Non-ribosomal peptide synthetases are important enzymes for the assembly of complex peptide natural products. Within these multi-modular assembly lines, condensation domains perform the central function of chain assembly, typically by forming a peptide bond between two peptidyl carrier protein (PCP)-bound substrates. To address this, we report the structure and biochemical characterization of complexes of a PCP domain bearing a stable analog of the acyl acceptor complexed to the acceptor site of a C domain from the NRPS that biosynthesizes fuscachelin in the thermophile Thermobifida fusca. The C3 domain of the didomain resembles other members of its class, comprising a pseudo-dimer of CAT domains with bridge (R2923 to T2944) and floor loop (A2843 to L2858) regions.

The crystals belonged to the P212121 space group, with the unit cell comprising two highly similar copies of the PCP2-C3 construct (RMSD (all atoms) 0.74 Å). In the PCP2-C3 didomain structure, the PCP2 domain sits at the acceptor-PCP binding site (near the opening of the acceptor substrate channel) on the C3 domain from the second chain in the asymmetric unit. The interface between the PCP2 domain and C3 domain is mostly hydrophobic in nature (537/510 Å2 buried surface area (chain A/B) excluding PPant), with the side chains of V2534, L2515, L2518, F2508, and F2538 of the PCP domain playing a major role in the interaction along with residues A2907, V2908, V2584, L2580, and W2579 of the C domain. We were surprised, therefore, to find that this construct crystallized with the PCP2 domain positioned at the acceptor-PCP binding site of the C3 domain of the second chain in the asymmetric unit. Mass spectrometric analysis of the PCP2-C3 didomain construct revealed a 340 Dalton mass increase, consistent with attachment of PPant to S2514, likely installed by the phosphopantetheinyl transferase EntD that phosphopantetheinylates some PCP domains when they are expressed in E. coli. Having confirmed the presence of a PPant arm, we modeled this into the electron density observed in our structure. Interestingly, we found that this did not extend into the active site of the C domain, but instead curled back towards the outer surface of the C domain. The side chain of R2577 appears to block the channel that leads to the active site of the C domain. Access of the PPant arm to the C domain active site appears to be gated by R2577, which repels the unmodified PPant arm (or neutral/negatively charged substrates) in favor of the aminoacyl-PPant.

>[2x]VTAYEEIVCQVFAAVLDRSDVTADADFFALGGHSLLSLRVVARLRALLGVDVGVRDLFEAPTPAALAARLTTQTGRRPAVTRRGPDAPPVLSHFQRRLWLIEQVYQTRGAYNVPLAVHVSDRLDLDVLRAAVRDLVARHEVLRTLVRSSDDGPDPVLLAPEDAAVDVAEVQAAGPVADLLAELTAQPFDLATQIPLRVRMITGEQVDGCVLLLVCHHIAADEWSFAPLLRDLDTAYRARAAGRAPDWEPLPAQYSDYAATLHDWLGEATDPASPLRRQLDYWQHALQDLPDELDLPTDRPRPATASHRGGLARAELPPELVEAVRRLAAQHGVTVFMVVQAAVAVLLHRLGAGDDIPLGSPVADRADEAVHDTVGFFLNTLVLRVNLSGNPTFADLLDRVRAVDLEAFARADAPFDAVVDTVKPPRAVSRHPLFQTMVSYQRRPSDVDRLFGAATRLVEVPLDTAKFDLEFAFIEDGHGGAHIALNYAADLFDHDSAEQLVARLRTVLEHACADPCRPVAGVEVVSGA> MNVGTAHSEVNPNTRVMNSRGIWLSYVLAIGLLHIVLLSIPFVSVPVVWTLTNLIHNMGMYIFLHTVKGTPFETPDQGKARLLTHWEQMDYGVQFTASRKFLTITPIVLYFLTSFYTKYDQIHFVLNTVSLMSVLIPKLPQLHGVRIFGINKY;>MATATEQWVLVEMVQALYEAPAYHLILEGILILWIIRLLFSKTYKLQERSDLTVKEKEELIEEWQPEPLVPPVPKDHPALNYNIVSGPPSHKTVVNGKECINFASFNFLGLLDNPRVKAAALASLKKYGVGTCGPRGFYGTFDVHLDLEDRLAKFMKTEEAIIYSYGFATIASAIPAYSKRGDIVFVDRAACFAIQKGLQASRSDIKLFKHNDMADLERLLKEQEIEDQKNPRKARVTRRFIVVEGLYMNTGTICPLPELVKLKYKYKARIFLEESLSFGVLGEHGRGVTEHYGINIDDIDLISANMENALASIGGFCCGRSFVIDHQRLSGQGYCFSASLPPLLAAAAIEALNIMEENPGIFAVLKEKCGQIHKALQGISGLKVVGESLSPAFHLQLEESTGSREQDVRLLQEIVDQCMNRSIALTQARYLEKEEKCLPPPSIRVVVTVEQTEEELERAASTIKEVAQAVLL[2x];> MADYKDDDDKSGPDEVDASGRMAGMALARAWKQMSWFYYQYLLVTALYMLEPWERTVFNSMLVSIVGMALYTGYVFMPQHIMAILHYFEIVQ;> MRPEPGGCCCRRTVRANGCVANGEVRNGYVRSSAAAAAAAAAGQIHHVTQNGGLYKRPFNEAFEETPMLVAVLTYVGYGVLTLFGYLRDFLRYWRIEKCHHATEREEQKDFVSLYQDFENFYTRNLYMRIRDNWNRPICSVPGARVDIMERQSHDYNWSFKYTGNIIKGVINMGSYNYLGFARNTGSCQEAAAKVLEEYGAGVCSTRQEIGNLDKHEELEELVARFLGVEAAMAYGMGFATNSMNIPALVGKGCLILSDELNHASLVLGARLSGATIRIFKHNNMQSLEKLLKDAIVYGQPRTRRPWKKILILVEGIYSMEGSIVRLPEVIALKKKYKAYLYLDEAHSIGALGPTGRGVVEYFGLDPEDVDVMMGTFTKSFGASGGYIGGKKELIDYLRTHSHSAVYATSLSPPVVEQIITSMKCIMGQDGTSLGKECVQQLAENTRYFRRRLKEMGFIIYGNEDSPVVPLMLYMPAKIGAFGREMLKRNIGVVVVGFPATPIIESRARFCLSAAHTKEIL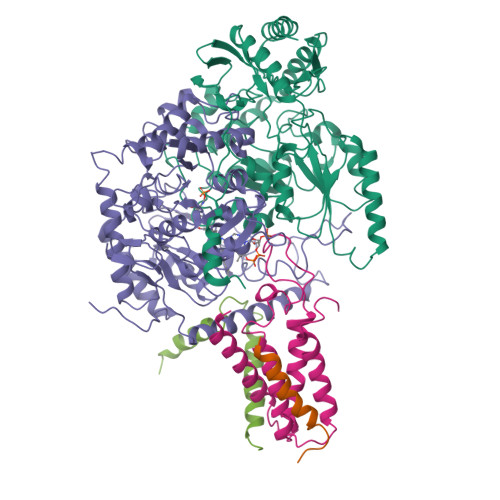DTALKEIDEVGDLLQLKYSRHRLVPLLDRPFDETTYEETED> AFPDCANGPLKSNLVCNASADPVSRAKALVDALTLEELVNNTVNASPGVPRVGLPPYNWWSEALHGVARSPGTNFSTVPGSPFSSATSFPQPIILGATFDDDLIHSIATVISTEARAFNNAGRAGLDFFTPNINPFKDPRWGRGQETPGEDPYHIAQYVYQLITGLQGGLSPDPYYKVVADCKHFAGYDLEDWHGNNRMAFNAVISTQDLAEFYTPSFQSCVRDAHVGSVMCSYNAVNGVPSCASPYLLQDLIRDHFGLGDGWITSDCDAVDNVFDPHNYTSTLVNASAVSLKAGTDVDCGTTYSQTLVDAVNQKLVTEDDVKTSMVRLYSSLVRLGYFDSPENQPWRQLGWADVNTPSAQALALTAAEEGVVLLKNDGTLPLSRRIKHIAVVGPWANATTQMQGNYQGIAPFLISPLQALQDAGFHVSFANGTAINSTDTSGFASALMAAKAADAIVFAGGIDETIESEGHDRDSIEWPGNQLDLIEQLAALRKPLIVLQMG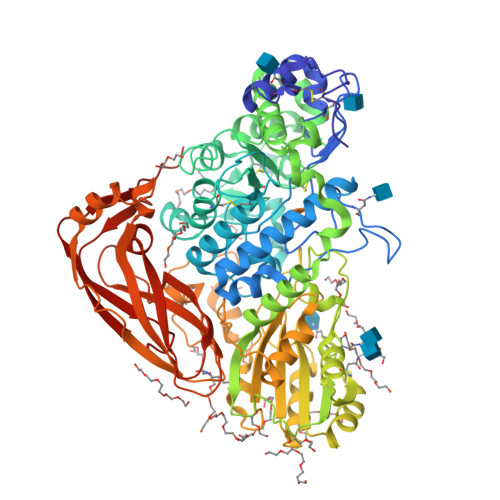GGQVDSSSLKASKAVNALLWGGYPGQSGGTAIVNILTGKTAPSGRLPITQYPAAYVDAIPMTDMALRPSSSSPGRTYKWYTGTPVFDFGFGLHYTSFKLSWAASPPSRFDISSLVAGAKHAGVAFTDLAPLFTFHVAVKNSGKVTSDYVALLFAHTTVGPSPAPQQELVAYTRVKGITPGRTATAALSVTLGSIARVDESGVRSLYPGKYSVWVDTTREIMHTFELTGKTTQILGWPQPR> MASAHIALELDKTKVKVGDVIVATVKAKNMTSMAGIQVNIKYDPEVLQAIDPATGKPFTKETLLVDPELLSNREYNPLLTAVNDIN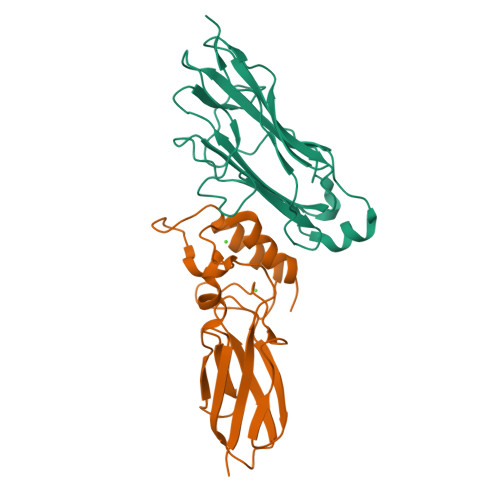SGIINYASCYVYWDSYRESGVSESTGIIGKVGFKVLKAANTTVKLEETRFTPNSIDGTLVIDWYGQQIVGYKVIQPDLEHHHHHH;> MNNDSTDKTTVSGYISVDFDYPPESESKIKSGFNVKVAGTELSTKTDEKGYFEISGIPGDMREFTLEISKRNYLKRNVTVNGTGKLVVSTEDNPLILWAGDVERKGVQDNAINMVDVMEISKVFGTRAGDEEYVAELDLNMDGAINLFDIAIVIRHFNALPSRY> MESKNKTAATQQSEPNVIAAHKGVNQAPVPLKMERVGPHDVHIEMTAQITDIEIDKGKIYKAWTFNGQAPGPLVVVNEGDTIHFTLKNMDPVVPHSMDFHAVH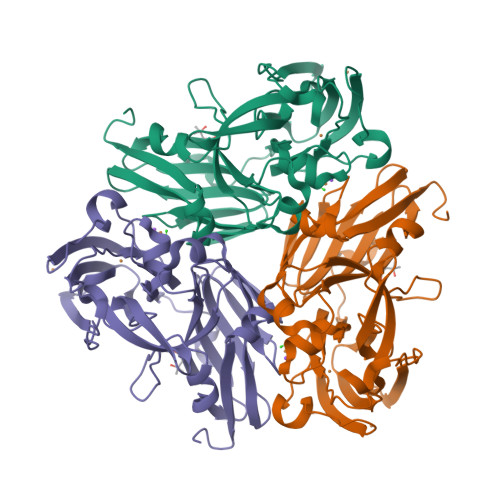ASPSKDFIDVMPNKSGTFTYPANKPGVFMYHCGTKPVLQHIANGMHGVIIVKPKNGYPTDKEVDREYVLIQNEWYKYNDMNDFQNGVPSYVVFSSKALKPGDPNTNGDTFTLKEKPLLAKVGEKIRLYINNVGPNEVSSFHVVGTVFDDVYLDGNPNNHLQGMQTVMLPASGGAVVEFTVTRPGTYPIVTHQFNHAQKGAVAMLKVTETGEDDGTETSGH> ASTQGISEDLYNRLVEMATISQAAYADLCNIPSTIIKGEKIYNAQTDINGWILRDDTSKEIITVFRGTGSDTNLQLDTNYTLTPFDTLPQCNDCE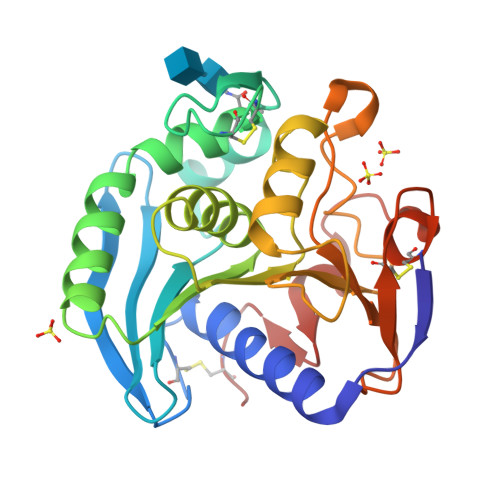VHGGYYIGWISVQDQVESLVKQQASQYPDYALTVTGHSLGASMAALTAAQLSATYDNVRLYTFGEPRSGNQAFASYMNDAFQVSSPETTQYFRVTHSNDGIPNLPPADEGYAHGGVEYWSVDPYSAQNTFVCTGDEVQCCEAQGGQGVNDAHTTYFGMTSGACTW Here, we report three Pb2+-complexed structures of the thrombin binding aptamer (TBA). These high-resolution crystal structures showed that TBA forms intramolecular G-quadruplex and Pb2+ is bound by the two G-tetrads in the center. Each TBA molecule folds into an antiparallel chair-like quadruplex, which can be divided into four regions: two TT linkers (T3T4 and T12T13), one TGT linker (T7G8T9) and the central G-tetrads. The Pb2+ ion resides in-between the two G-tetrads, coordinating with the eight O6 atoms of the G-tetrads.

The B-form structure belongs to the orthorhombic space group P212121; per asymmetric unit contains six TBA-Pb2+ complexes. As calculated by the Matthews Coefficient program, the solvent content (44.7%) of the A-form structure is higher than that (40.0%) of the B-form structure. In fact, the six TBA-Pb2+ complexes within the asymmetric unit of the B-form structure also assembled into dimers: dimer AB, CD and EF. The overall fold of the AB and CD dimers is very similar to that of the A-form structure. The overall fold of the EF dimer is also very similar to other dimers, but the relative orientation of the EF dimer is different from others. When the EF dimer is superimposed with the AB dimer of the A- or B-form structure, there is one 180° rotation (along the central vertical axis) between the F and B molecules. T3, T4, T12 and T13 also arrange in two layers in the EF dimer of the B-form structure. However, due to the rotation of the F molecule, T3 and T4 of molecule F interact with T4 and T3 of molecule E, respectively. Likewise, T12 and T13 of the two molecules interact with each other. The average Pb2+–O6 coordinating distance is only 2.65 Å in the A-form TBA-Pb2+ complex structure. Similar Pb2+–O6 coordination and coordinating distance are also observed in the B-form TBA-Pb2+ complex structure.

>GGTTGGTGTGGTTGG[6x]> MRLPDAGFRRYIV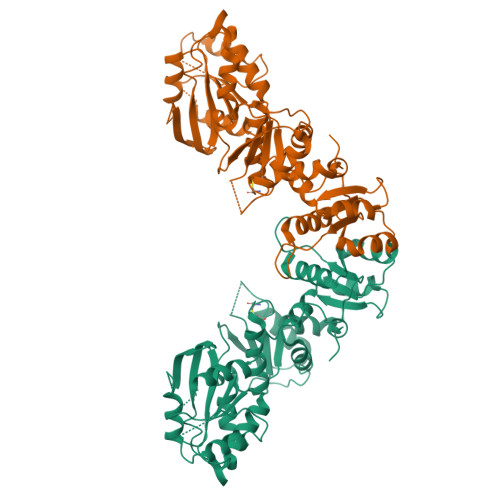VAGRRNVGKSSFMNALVGQNVSIVSEYAGTTTDPVYKSMELYPVGPVTLVDTPGLDDVGELGRLRVEKARRVFYRADCGILVTDSEPTPYEDDVVNLFKEMEIPFVVVVNKIDVLGEKAEELKGLYESRYEAKVLLVSALQKKGFDDIGKTISEILPGDEEIPYLGDLIDGGDLVILVVPIDLGAPKGRLIMPQVHAIREALDREAIALVVKERELRYVMENIGMKPKLVITDSQVVMKVASDVPEDVELTTFSIVESRYRGDLAYFVESVRKIEELEDGDTVVIMEGCTHRPLTEDIGRVKIPRWLVNHTGAQLNFKVIAGKDFPDLEEIEGAKLIIHCGGCVLNRAAMMRRVRMAKRLGIPMTNYGVTISYLHGVLDRAIRPFREEVKV FLUORESCEINYLTHIOUREIDO | 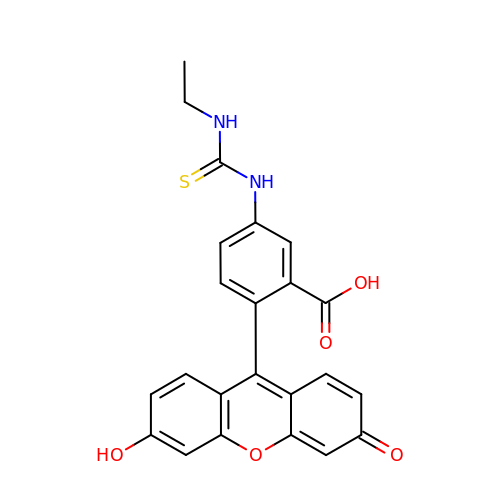C23 H18 N2 O5 S | VHJFQSRUDVDTEO-UHFFFAOYSA-N>GLVPRGSHMAKHLFTSESVSEGHPDKIADQISDAVLDAILEQDPKARVACETYVKTGMVLVGGEITTSAWVDIEEITRNTVREIGYVHSDMGFDANSCAVLSAIGKQSPDINQGVDRADPLEQGAGDQGLMFGYATNETDVLMPAPITYAHRLVQRQAEVRKNGTLPWLRPDAKSQVTFQYDDGKIVGIDAVVLSTQHSEEIDQKSLQEAVMEEIIKPILPAEWLTSATKFFINPTGRFVIGGPMGDCGLTGRKIIVDTYGGMARHGGGA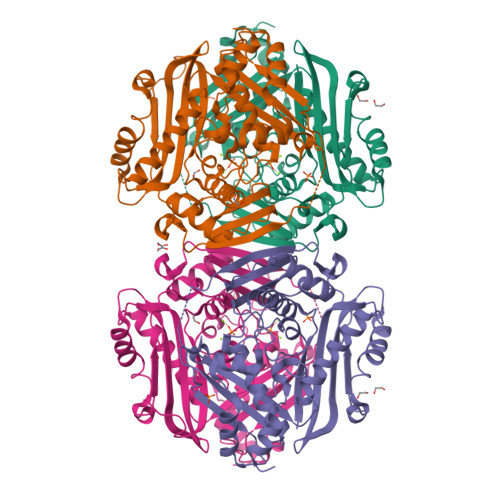FSGKDPSKVDRSAAYAARYVAKNIVAAGLADRCEIQVSYAIGVAEPTSIMVETFGTEKVPSEQLTLLVREFFDLRPYGLIQMLDLLHPIYKETAAYGHFGREHFPWEKTDKAQLLRDAAGLK[2x]> MALTLPKGIVFGFAPITSTTSSVTGVTRAAPPVATGTMLTAGTTVLVRSNTWTGINNRISVVDANKALQGFDTTDTTTYPGTSGPVELITVGAFVNFTQQGEPSTSGGDQQFWNGQLLEDRSGRQLAIPTFKNAK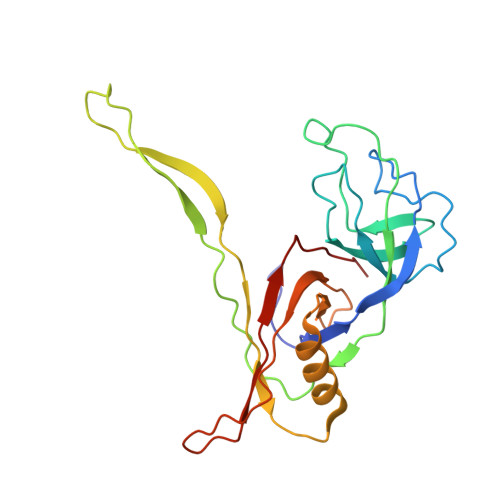TLTLPLYMDTSLPWYAAAKAADARGEPVAVRMLLPNGDASYNYGYMSFDGDATITANAPITNVATFTFLSDSTLVEA>MASMTGSAKLISVTKPVVEGVNTAEELIAYAARVSNPENQINNKTASGLLKYCIRHKHWSIFETAFMTLELKTSRGIAAQVLRHRSFHFQEFSQRYASVMETPPPHQARFQDHKNRQNSLDTVPEDDQTWWATEQEKLYAQSMELYNKALEKGIAKE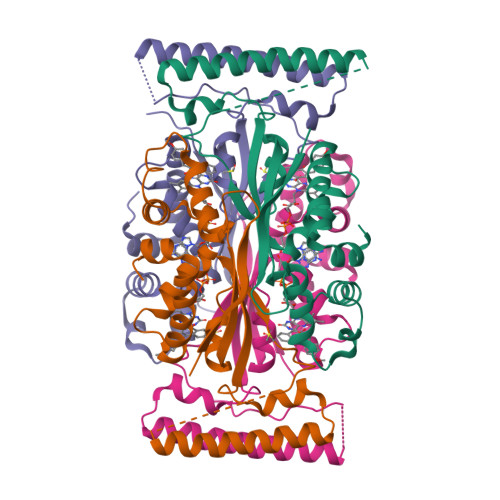CARFILPLSTPTTIYMSGTIRDWIHYIELRTSNGTQREHIDLANACKEIFIKEFPSIAKALDWVHHHHHH[16x]>MTLSKIKLFYNTPFNNMQNTLHFNSNEERDAYFNSKFDVHEFTSTFNYRNMKGVLRVTIDLVSDRSCFEQLMGVNYCQVQYIQSNRVEYLFVTDIQQLNDKVCELSLVPDVVMTYTQGNVLNTLNNVNVIRQHYTQTEYEQNLEQIRSNNDVLATSTMRVHAIKSELFTQLEYILTIGANLRKSFGTAEKPKFPSSSGSTHDGIYNPYDMYWFNDYESLKEVMDYLTGYPWIQQSIKNVTIIPSGFIKQESLNDHEPVNGGDLSVRKLGKQGVSNQKDFNAISLDYQSLMFTLGLNPINDKHLLRPNIVTAELTDYAGNRLPIDLSLIETNLEFDSFVTMGAKNEIKVYVKNYNARGNNVGQYIDNALTINNFDTIGFSVDSGELGKANSAYSRELSNSRQMSSRINTVLDNDASVKDRLFNAISLSGGLSIKSALSGFNNEYEHYRDQKAQFKQMDALPNAITEGHVGYAPLFKQDKFGVHLRLGRISQDELNNVKKYYNMFGYECNDYSTKLSDITSMSICNWVQFKGIWTLPNVDT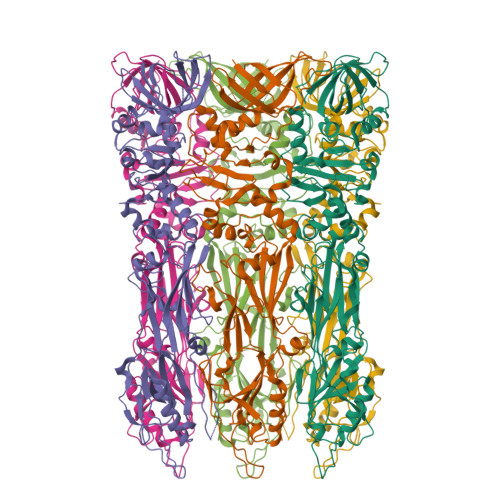GHMNMLRALFEAGVRLWHKESDMINNTVVNNVIIKSLEHHHHHH[12x]>MRIVVTGGAGFIGSHLVDKLVELGYEVVVVDIVQRDTGGSAELHVRDLKDYSWGAGIKGDVVFHFAANPEVRLSTTEPIVHFNENVVATFNVLEWARQTGVRTVVFASSSTVYGDADVIPTPEEEPYKPISVYGAAKAAGEVMCATYARLFGVRCLAVRYANVVGPRLRHGVIYDFIMKLRRNPNVLEVLGDGTQRKSYLYVRDAVEATLAAWKKFEEMDAPFLALNVGNVDAVRVLDIAQIVAEVLGLRPEIRLVPSTPDGRGWPGDVKYM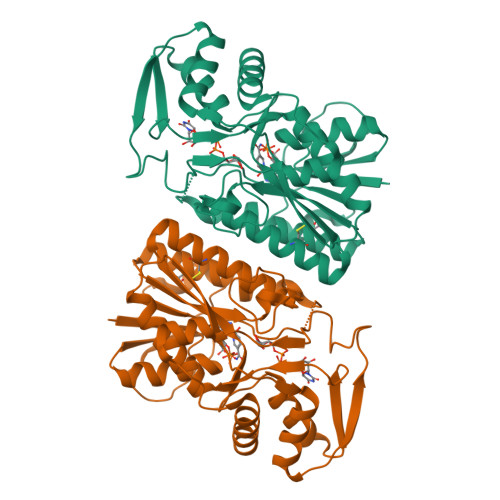TLAVTKLMKLTGWRPTMTSAEAVKKTAEDLAKELWG[3x]> SEHNEKGVLLKSSISFQNIIEGTRNFHKDFLIGEGEIFEVYRVEIQNLTYAVKLFKQEKKMQCKKHWKRFLSELEVLLLFHHPNILELAAYFTETEKFCLIYPYMRNGTLFDRLQCVGDTAPLPWHIRIGILIGISKAIHYLHNVQPCSVICGSISSANILLDDQFQPKLTDFAMAHFRSHLEHQSCTINMTSSSSKHLWYMPEEYIRQGKLSIKTDVYSFGIVIMEVLTGCRVVLDDPKHIQLRDLLRELMEKRGLDSCLSFLDKKVP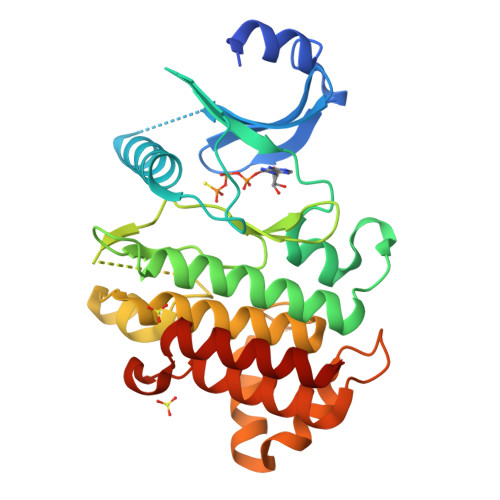PCPRNFSAKLFCLAGRCAATRAKLRPSMDEVLNTLESTQASLYFAED> SKTITIYLDHASLPTLNQLMHFTKESEDKETARIFGFSRFKLPEKITEQYNNIHFVEIKNNRPTEDIFTILDQYPEKLELDLHLNIAHSIQLFHPILQYRFKHPDRISIKSLNLYDDGTMEYVDLEKEENKDIKSAIKKAEKQLSDYLLTGKINFDNPTLARYVWQSQYPVKYHFLSTEYFEKAEFLQPLKTYLAGKYQKMDWSAYEKLSPEQQTFYLKLVGFSDETKQLFHTEQTKFIFTGTTTWEGNTDIREYYAKQQLNLLKHFTHSEGDLFIGDQYKIYFKGHPR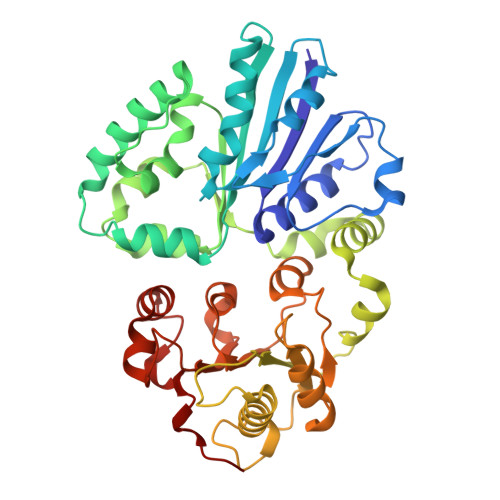GGDINDYILKHAKDITNIPANISFEILMMTGLLPDKVGGVASSLYFSLPKEKISHIIFTSNKKIKNKEDALNDPYVRVMLRLGMIDKSQIIFWDSLKQL> SFSSPSGSTIEAGIAYPISTGFDPLTSSGASSMAANLHIFEGLVDLHPVTRQPYLALAAKEPEQKDDLTYYISLREGAMFHDGSPVTTEDVVYSFERVLDPAKASLFAQFIPFIASVTALDDNVVEFKLKYPFALFKERLTIIKIVPKHIVEAGQSAFDAKPIGSGPYKFVSATKDDRIVFEANTVYNGHYPAKVEKMTWFLLSDDAARVTAQESGRVQAIESVPYLDAERLKRKNNVESVQSFGLLFLMFNCEKAPFDNPKVRQALHYALDKQKLIDIVFLGNAKAATSYLQDTHPDYVKASSQYDYDKAKAEKLLAEAGITNLTFQLLATDHAWVKECAPLILESWNALSVVKVTLQHLQSGALYSAHVDKGAYEVVIAPGDPSVFGNDLDLLLSWW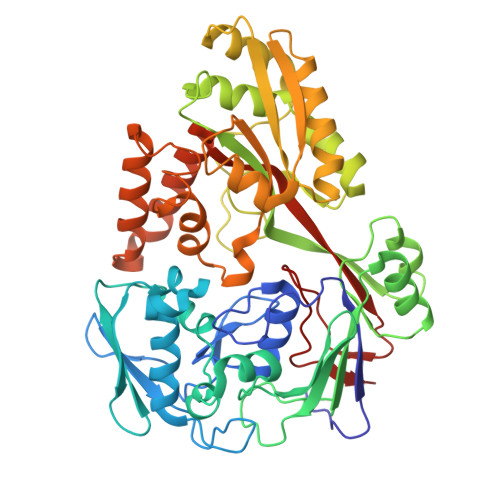YRGDVWPKRRFRWANTAEYHEVQKLLDEAIKNPAGSKVAWQKAINIIAEQVPLYPIIHRKLPTAWNTKKLTDFQPLPTTGLSFLGVGRT Reversal of PARylation is predominantly carried out by poly(ADP-ribose) glycohydrolase (PARG) in nucleus and cytosol, whereas ADP-ribosylhydrolase 3 (ARH3) may play a role in mitochondrial PAR degradation. PARG comprises an N-terminal regulatory/targeting domain and a C-terminal catalytic domain. The mouse PARG catalytic domain has a bean-shaped structure, with the active site in a deep cleft in the middle on the abdominal side.

To understand what caused the activity difference between the mPARG E748N/Q and E749N/Q mutants, we solved the crystal structures of these mPARG mutants. Interestingly, while E748N and E749N mutants were completely dead, both E748Q and E749Q mutants still retained residual PARG activities. PARG E748Q and E749Q mutants have very similar conformation in the active site, consistent with the fact that glutamine has the similar size of side chain with glutamate. To study the enzymatic mechanism of mPARG, we tried to soak the catalytic residue Glu748, Glu749 mutants E748N, E748Q, E749N and E749Q with the iso-ADPr, which may be the smallest PARG substrate containing the α(1→2) ribose-ribose glycosidic bond to be cleaved by PARG. In all above four PARG mutant crystal structures, we were not able to observe the electron density for iso-ADPr at the “active” site of mPARG. For the E748Q and E749Q mutants, this may result from the partial catalytic activities of these mutations and/or the low affinity between PARG and iso-ADPr. Surprisingly, we repeatedly observed electron densities, in an unexpected position, which fit well with the chemical structure of iso-ADPr and refined well when iso-ADPr was built into the densities. In these structures, iso-ADPr sits at the secondary binding site which is far away from the cleft. This secondary binding site is at the mouse PARG exon 5 coded region, and is not formed due to crystal packing as it is far away from any PARG region involved in crystal packing. There are four residues (R478, D480, F491 and T493) directly interacting with iso-ADPr.

> GNLPPEKKWLGTPIEEMRKMPRCGIHLPSLRPSASHTVTVRVDLLRAGEVPKPFPTHYKDLWDNKHVKMPCSEQNLYPVEDENGERTAGSRWELIQTALLNKFTRPQNLKDAILKYNVAYSKKWDFTALVDFWDKVLEEAEAQHLYQSILPDMVKIALCLPNICTQPIPLLKQKMNHSVTMSQEQIASLLANAFFCTFPRRNAKMKSEYSSYPDINFNRLFEGRSSRKPEKLKTLFCYFRRVTEKKPTGLVTFTRQSLEDFPEWERCEKPLTRLHVTYEGTIEGNGRGMLQVDFANRFVGGGVTGAGLVQQEIRFLINPELIVSRLFTEVLDHNECLIITGTEQYSEYTGYAETYRWARSHEDGSEKDDWQRRCTEIVAIDALHFRRYLDQFVPEKVRRELNKAYCGFLRPGVPSENLSAVATGNWGCGAFGGDARLKALIQILAAAAAERDVVYFTFGDSELMRDIYSMHTFLTERKLDVGKVYKLLLRYYNEECRNCSTPGPDIKLYPFIYHAVESSAET>GPLGSPEFQKTKPFSVPNLPLNTLSNSRVPSLINAMMISRDHGQMVQFQNGRVTLDGQLQGTTPTSLSQLCKIRGKVFHASGGNGLNLTELDGSAYHAFESPAPIGFPDIGDCDWHMSATATNNFTGSSNEYQILIKQESAFAPHLGHVQADNLSAGANTDLIVSLSWISPVSDQHRHDVDPWVIPRYGSSLTEAAQLAPPIYPPGFGEAIVFFMSDFPVVSGVNGMRIPCTLPQEYVAHFVNEQAPTRGEAALLHYVDPDTHRNLGEFKMYPEGFMTCVPNSSGSGPQTLPINGVFTFVSWVSRFYQLKP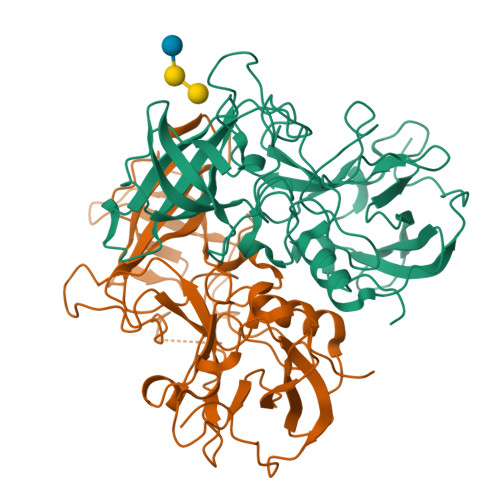VGTAGPARRLGIRRS[2x]> QMNYEEVIKKYRGEENFDHAAYDWRLHSGVTPVKDQKNCGSCWAFSSIGSVESQYAIRKNKLITLSEQELVDCSFKNYGCNGGLINNAFEDMIELGGICPDGDYPYVSDAPNLCNIDRCTEKYGIKNYLSVPDNKLKEALRFLGPISISVAVSDDFAFYKEGIFDGECGDQLNHAVMLVGFGMKEIVNPLTKKGEKH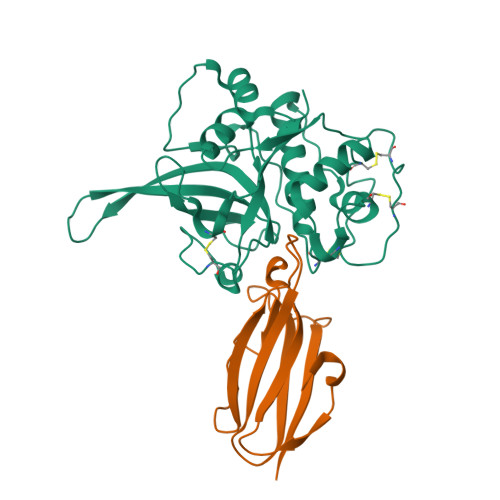YYYIIKNSWGQQWGERGFINIETDESGLMRKCGLGTDAFIPLIE;> MSHKVTKAHNGATLTVAVGELVEIQLPSNPTTGFAWYFEGGTKESPNESMFTVENKYFPPDSKLLGAGGTEHFHVTVKAAGTHAVNLTYMRPWTGPSHDSERFTVYLKAN>[2x]MLSHMVLTRQDIGRAASYYEDGADDYYAKDGDASEWQGKGAEELGLSGEVDSKRFRELLAGNIGEGHRIMRSATRQDSKERIGLDLTFSAPKSVSLQALVAGDAEIIKAHDRAVARTLEQAEARAQARQKIQGKTRIETTGNLVIGKFRHETSRERDPQLHTHAVILNMTKRSDGQWRALKNDEIVKATRYLGAVYNAELAHELQKLGYQLRYGKDGNFDLAHIDRQQIEGFSKRTEQIAEWYAARGLDPNSVSLEQKQAAKVLSRAKKTSVDREALRAEWQATAKELGIDFS

Relaxases are DNA strand transferases responsible for the initial and final stages of DNA processing during bacterial conjugation, a mechanism of DNA transfer between bacterial cells. TrwC is the relaxase of the prototype plasmid R388. It is a relaxase of the MOBF family, presently composed by 114 members and including relaxase TraI of plasmid F. TrwC presents two domains: relaxase and helicase. The relaxase domain is responsible for DNA recognition; it shows extremely high specificity towards its cognate nic-site.

Deeper analysis of the ssDNA region of the nic-site focused on the U-shaped turn located close to the catalytic site, which is conserved in the nic-site of the related plasmid F. We solved the X-ray structure of a TrwC nucleoprotein complex containing a nic-site mutant efficiently processed by TrwC that carries a different combination of nucleotides in the U-shaped turn. Nic-site mutants III, IV and V, are still efficiently transferred although they present 3–4 mutations around the cleavage site, affecting the nucleotides involved in the U-shaped structure. Moreover, although all previous TrwC structures were obtained with selenomethionine derivatives of TrwCR, we were able to obtain native crystals with TrwCR-mutant IV. The main difference revealed by the new structure was the formation of a different U-shaped structure, in which the formation of three hydrogen bonds between G22C and T25G in TrwCR-IV stabilize the U-turn shape DNA structure. In the IV mutant, both Lys262 and Ser89 interact now with G25 and Lys262 with T24. These protein–DNA interactions together with maintenance of the T23 interactions with the protein and the Watson–Crick base pairing between C22 and G25 allows the formation of the U-shape structure in TrwCR-IV. In the three dimensional (3D) structure of the TrwCR–MIV complex, there is an obvious new interaction, a triple hydrogen bond between C22 and G25 that makes the structure resemble in size and charge distribution of the U-shaped turn of the wt complex. In all MOBF structures, T23 is extruded from the extended ssDNA by its tight binding to the relaxase. The mutant IV containing scDNA is slightly less prone to in vitro relaxation by TrwC than the scDNA containing the wt nic-site, although TrwC can still relax mutant IV scDNA. TrwC is able to cleave a mutant IV-containing oligonucleotide RIV(25 + 18).>[6x]MGSSHHHHHHGSNAWEVNFDGLVGLTHHYAGLSFGNEASTRHRFQVSNPRLAAKQGLLKMKALADAGFPQAVIPPHERPFIPVLRQLGFSGSDEQVLEKVARQAPHWLSSVSSASPMWVANAATIAPSADTLDGKVHLTVANLNNKFHRSLEAPVTESLLKAIFNDEEKFSVHSALPQVALL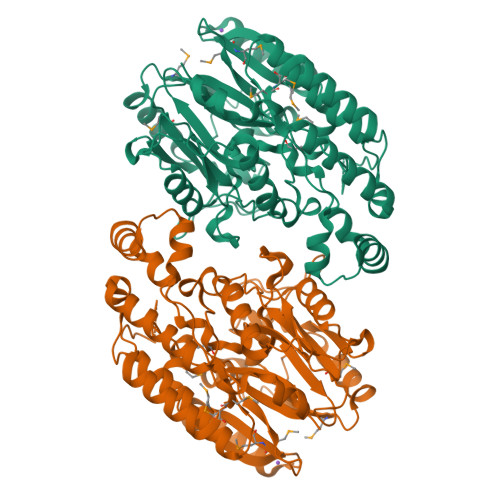GDEGAANHNRLGGHYGEPGMQLFVYGREEGNDTRPSRYPARQTREASEAVARLNQVNPQQVIFAQQNPDVIDQGVFHNDVIAVSNRQVLFCHQQAFARQSQLLANLRARVNGFMAIEVPATQVSVSDTVSTYLFNSQLLSRDDGSMMLVLPQECREHAGVWGYLNELLAADNPISELKVFDLRESMANGGGPACLRLRVVLTEEERRAVNPAVMMNDTLFNALNDWVDRYYRDRLTAADLADPQLLREGREALDVLSQLLNLGSVYPFQREGGGNG>MTNIEILENMLKLQQKLNDETNGLNWENGYTKEGKLISWRRCIYMECAELIDSFTWKHWKNISSLTNWENVRIEIVDIWHFILSLLLEEYRDKNNKDFKAIATEVNAVSVFQDFCKEEEYPNEGDIYGILNDIELIIHKCSGFGFNLGELLSTYFTLAI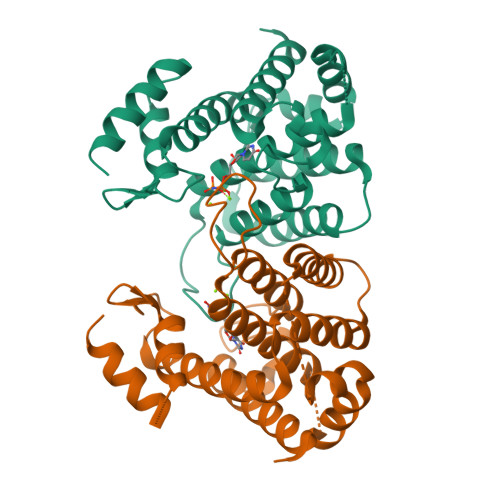KCGLNLEILYKTYIGKNVLNIFRQNNGYKDGSYKKTWNGKEDNEVLAQILEQELDFDTIYKKLEECYKKA[2x]> MATLAFILYKYFPF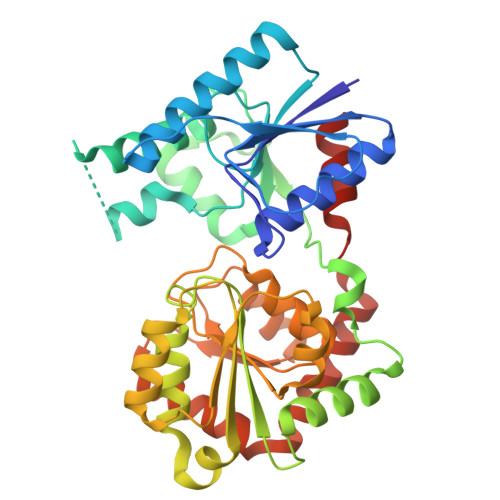GGLQRDFMRIALECQRRGHDIRVYTLIWEGDVPDGFEVLVAPVRSIFNHRRNEKFTAWVRADLDRRPVQRVIGFNKMPGLDVYYAADACFEEKAQTLRNPLYRQWGRYRHFAGYERAVFDPASKTEILMISEVQQPLFVKHYGTQAERFHLLPPGISQDRRAPANAADVRAEFRREFGLEEDDLLLVQIGSGFKTKGLDRSLKALSALPKALRRRTRLIAIGQDDPKPFLLQIAALGLNDQVQILKGRSDIPRFLLGADLLIHPAYNENTGTVLLEALVSGLPVLVTDVCGYAHYIAEADAGRVLPSPFEQDSLNRLLAEMLEDAPARAAWSRNGLAYADHADLYSMPQRAADLILGEAS> DAIADASKRFSDATYPIAEKFDWGGSSAIAKYIADASAG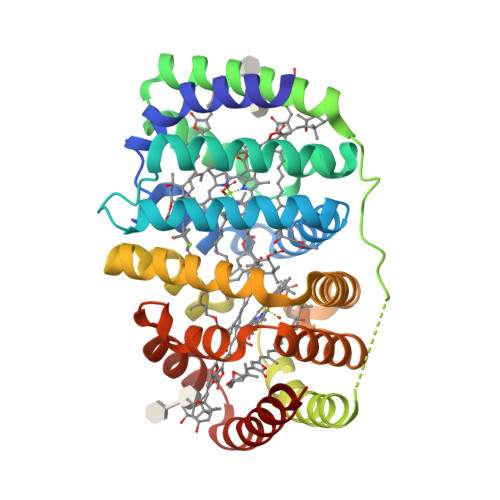NPRQAALAVEKLLEVGLTMDPKLVRAAVEAHSKALDSAKKNAKLMASKEDFAAVNEALARMIASADKQKFAALRTAFPESRELQGKLFAGNNAFEAEKAYDSFKALTSAVRDASINGAKAPVIAEAARAERYVGDGPVGRAAKKFSEATYPIMDKLDWGKSPEISKYIETASAKNPKMMADGIDKTLEVALTMNQNAINDAVFAHVRAIKGALNTPGLVAERDDFARVNLALAKMIATADPAKFKALLTAFPGNADLQMALFAANNPEQAKAAYETFVALTSAVASST>[4x]GPYASLTEIEHLVQSVCKSYRETCQLRLEDLLRQRSNIFSREEVTGYQRKSMWEMWERCAHHLTEAIQYVVEFAKRLSGFMELCQNDQIVLLKAGAMEVVLVRMCRAYNADNRTVFFEGKYGGME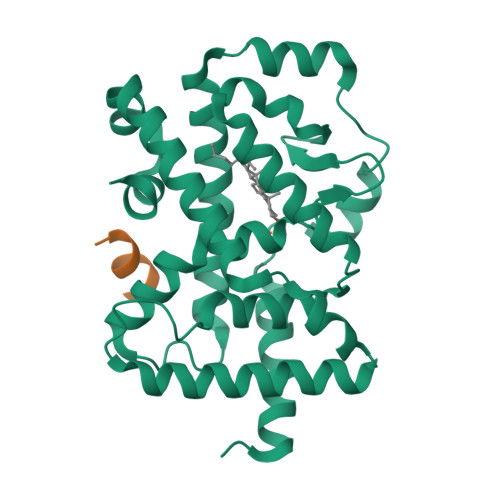LFRALGCSELISSIFDFSHSLSALHFSEDEIALYTALVLINAHRPGLQEKRKVEQLQYNLELAFHHHLSKTHRQSILAKLPPKGKLRSLCSQHVERLQIFQHLHPIVVQAAFPPLYKELFSTETESPVGLSK;>[4x]NSHQKVTLLQLLLGHKNEEN> GHMHNAEAIPQEPMDLENLDSEKRAARIAAGTIIAGAELTIGLLQNLLDVLANVNRKCAVGVDNESGFRWQEGSTYFFSGTADENLPYSVSDGYAVLYGPRKTNGPVATGVVGVLAYYIPSIGKTLAVMWSVPFDYNFYQNWWNAKLYSGNQDADY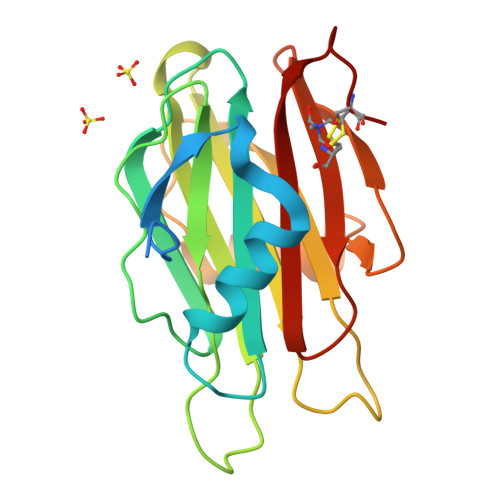DHYVDLYYDANPFKANGWHERSLGSGLKFCGSMSSSGQATLEIHVLKESETCM TRPV6 is a representative of the vanilloid subfamily of transient receptor potential (TRP) channels that serves as an entry gate for capturing dietary calcium ions in the gut1–3. In a nutshell, hTRPV6 is assembled of four subunits and contains a transmembrane domain (TMD) with a central ion channel pore and an intracellular skirt that is mostly built of ankyrin repeat domains connected by the three-stranded β-sheets, N-terminal helices, and C-terminal hooks. The TMD is composed of six transmembrane helices S1–S6 and a re-entrant pore loop (P-loop) between S5 and S6. As in all representatives of the tetrameric ion channel family, the ion-conducting pore of TRPV6 has two narrow regions, the selectivity filter formed by the extended regions of the P-loop and the gate formed by the S6 bundle crossing, separated by the central cavity in the middle.

The second, predominant population of particles yielded a 2.66-Å 3D reconstruction with no symmetry imposed (C1), which had two densities of the size of a genistein molecule that had never been seen in TRPV6 reconstructions before. Further analysis showed that this second reconstruction represents a genistein-bound inhibited state of the channel, hTRPV6GEN. In contrast to hTRPV6Open, the gate region in hTRPV6GEN is narrow and fully sealed by the side chains of L574 and M578. Overall, the structure is ~4-fold symmetrical but shows noticeable deviations from the 4-fold symmetry at the intracellular region of the ion channel pore, around the two putative sites of genistein binding. Close inspection of the hTRPV6GEN cryo-EM map revealed two densities of the shape of a genistein molecule at the intracellular half of the ion channel pore that were not present in the hTRPV6Open map. The upper site (1) is located above the gate, at the bottom of the central cavity, and is contributed by the S6 hydrophobic residues M570, L571 and L574. The bottom site (2) is right below the gate, at the intracellular entrance to the ion channel pore, and contributed by the residues M578, G579, H582, W583 and A586. Two strong densities at the pore intracellular entrance, located two-fold symmetrically relative to the central pore axis, are observed in the cryo-EM density of hTRPV6GEN. Each of these densities is in the middle of three-histidine clusters, which include H587 of the B/D diagonal subunits pair as well as H582 and H587 of the A/C diagonal subunits pair. When binding to the open TRPV6 channel perpendicularly to the central pore axis, genistein molecules pull one diagonal pair of subunits (A/C) asymmetrically towards the channel center.

>[4x]MGLSLPKEKGLILCLWSKFCRWFQRRESWAQSRDEQNLLQQKRIWESPLLLAAKDNDVQALNKLLKYEDCKVHQRGAMGETALHIAALYDNLEAAMVLMEAAPELVFEPMTSELYEGQTALHIAVVNQNMNLVRALLARRASVSARATGTAFRRSPCNLIYFGEHPLSFAACVNSEEIVRLLIEHGADIRAQDSLGNTVLHILILQPNKTFACQMYNLLLSYDRHGDHLQPLDLVPNHQGLTPFKLAGVEGNTVMFQHLMQKRKHTQWTYGPLTSTLYDLTEIDSSGDEQSLLELIITTKKREARQILDQTPVKELVSLKWKRYGRPYFCMLGAIYLLYIICFTMCCIYRPLKPRTNNRTSPRDNTLLQQKLLQEAYMTPKDDIRLVGELVTVIGAIIILLVEVPDIFRMGVTRFFGQTILGGPFHVLIITYAFMVLVTMVMRLISASGEVVPMSFALVLGWCNVMYFARGFQMLGPFTIMIQKMIFGDLMRFCWLMAVVILGFASAFYIIFQTEDPEELGHFYDYPMALFSTFELFLTIIDGPANYNVDLPFMYSITYAAFAIIATLLMLNLLIAMMGDTHWRVAHERDELWRAQIVATTVMLERKLPRCLWPRSGICGREYGLGDRWFLRVEDRQDLNRQRIQRYAQAFHTRGSEDLDKDSVEKLELGCPFSPHLSLPMPSVSRSTSRSSANWERLRQGTLRRDLRGIINRGLEDGESWEYQI> GSMRHERVV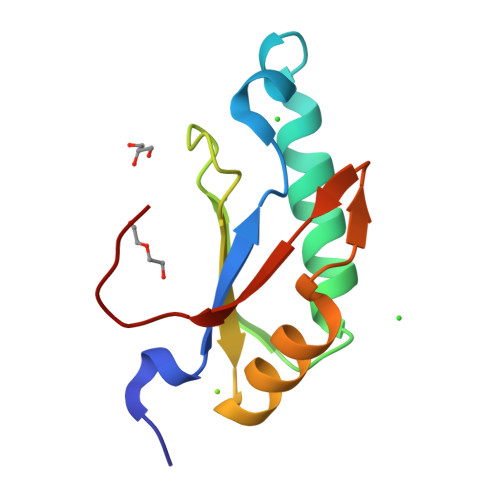IIKNMFHPMDFEDDPLVLNEIREDLRVECSKFGQIRKLLLFDRHPDGVASVSFRDPEEADYCIQTLDGRWFGGRQITAQAWDGTTDY>XAAAALAAALAQALX[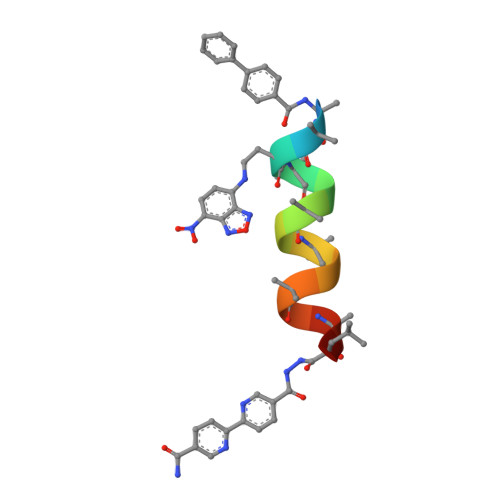4x]>MKAHPKEMVPLMGKRVAAPSGNPAILPEKRPAEITPTKKSAHFFLEIEGFEPNPTVAKTSPPVFSKPMDSNIRQCISGNCDDMDSPQSPQDDVTETPSNPNSPSAQLAKEEQRRKKRRLKKRIFAAVSEGCVEELVELLVELQELCRRRHDEDVPDFLMHKLTASDTGKTCLMKALLNINPNTKEIVRILLAFAEENDILGRFINAEYTEEAYEGQTALNIAIERRQGDIAALLIAAGADVNAHAKGAFFNPKYQHEGFYFGETPLALAACTNQPEIVQLLMEHEQTDITSRDSRGNNILHALVTVAEDFKTQNDFVKRMYDMILLRSGNWELETTRNNDGLTPLQLAAKMGKAEILKYILSREIKEKRLRSLSRKFTDWAYGPVSSSLYDLTNVDTTTDNSVLEITVYNTNIDNRHEMLTLEPLHTLLHMKWKKFAKHMFFLSFCFYFFYNITLTLVSYYRPREEEAIPHPLALTHKMGWLQLLGRMFVLIWAMCISVKEGIAIFLLRPSDLQSILSDAWFHFVFFIQAVLVILSVFLYLFAYKEYLACLVLAMALGWANMLYYTRGFQSMG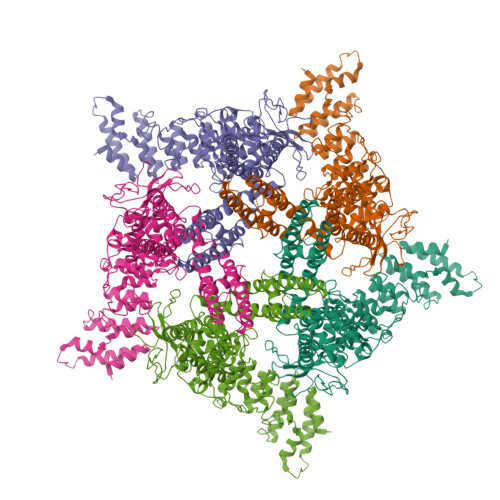MYSVMIQKVILHDVLKFLFVYIVFLLGFGVALASLIEKCPKDNKDCSSYGSFSDAVLELFKLTIGLGDLNIQQNSKYPILFLFLLITYVILTFVLLLNMLIALMGETVENVSKESERIWRLQRARTILEFEKMLPEWLRSRFRMGELCKVAEDDFRLCLRINEVKWTEWKTHVSFLNEDPGPVRRTDFNKIQDSSRNNSKTTLNAFEEVEEFPETSVLEVLFQGPWSHPQFEK[5x]>[2x]GSHHHHHHSQDPMKTQPNKTVIKILGLKNSKAASNPDGGLRSLLDFLERKSKEKITLGRGIIDGDYVWLKVNKDDAQHLLRLNGFTYAGATLTIEETNEPMPALSSQSKLSQAAQETKQKL

The Mex67–Mtr2 complex (NXF1–NXT1 in metazoans and small bristles in Drosophila melanogastor) is the principal mRNA-export factor in Sacccharomyces cerevisiae. Mex67/NXF1 is a modular protein constructed from four domains: an RNA-recognition motif (RRM) domain, a leucine-rich repeat (LRR) domain, a nuclear transport factor 2-like (NTF2L) domain and an ubiquitin-associated (UBA) domain. Mtr2 is a ∼15–20 kDa protein that also has an NTF2-like fold and forms a tight heterodimeric complex with the Mex67 NTF2L domain.

Like other NXF family members, ctMex67RRM did not contain a typical RRM consensus sequence that is based on two motifs: RNP1, (K/R)o-G-(F/Y)o-(G/A)i-Fo-Vi-Xo-(F/Y)i, and RNP2, (L/I)i-(Y/F)o-(V/I)i-(G/N)o-(G/N)o-(L/M)i, where the subscript ‘o’ or ‘i’ signifies whether the side chain is surface-exposed or facing the core of the RRM fold. In ctMex67RRM the RNP1 (residues 143–150) and RNP2 (residues 101–106) sequences were G-Do-Yo-Vi-Wo-Li-Ko-Vi and Ii-Ko-Ii-Lo-G-Li, respectively. The RNP2 motif appeared to be more conserved than RNP1, although the characteristic aromatic group at position 2 that typically forms ring-stacking interactions with RNA was instead lysine in ctMex67RRM. The large deviations from the RNP1 and RNP2 sequences found in different members of the NXF1/Mex67 family may reflect that they bind RNA in a more general, non-base-specific way, as appeared to be the case in the crystal structure of hsNXF1RRM-LRR–CTE-B, in which the hsNXF1 RRM domain formed mainly phosphate–backbone interactions with the CTE-B RNA. The UBA domain showed the greatest conservation (29% sequence identity over 55 residues), whereas the RRM domain had the lowest (15% identity over 73 residues). Classically, binding of the RNA cargo has been attributed to the RRM and LRR domains because together these domains are sufficient for Homo sapiens NXF1 to bind the viral RNA CTE (constitutive transport element) sequence motif.>LPCVPFSVAKSVKSLYLGRMFSGTPVIRLRFKRLQPTRLVAEFDFRTFDPEGILLFAGGHQDSTWIVLALRAGRLELQLRYNGVGRVTSSGPVINHGMWQTISVEELARNLVIKVNRDAVMKIAVAGDLFQPERGLYHLNLTVGGIPFHEKDLVQPINPRLDGCMRSWNWLNGEDTTIQETVKVNTRMQCFSVTERGSFYPGSGFAFYSLDYMRTPLDVGTESTWEVEVVAHIRPAADTGVLFALWAPDLRAVPLSVALVDYHSTKKLKKQLVVLAVEHTALALMEIKVCDGQEHVVTVSLRDGEATLEVDGTRGQSEVSAAQLQERLAVLERHLRSPVLTFAGGLPDVPVTSAPVTAFYRGCMTLEVNRRLLDLDEAAYKHSDITAHSCPPVEP[2x];>ESPFVSNPGNITGARGLTGTLRCQLQVQGEPPEVHWLRDGQILELVDSTQTQVPLGEDEQGDWIVASQLRITSLQ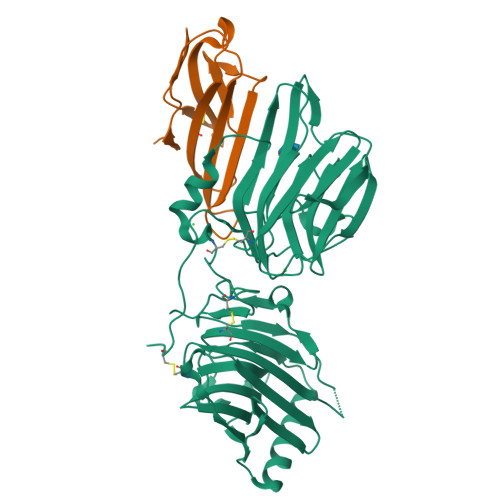LSDTGQYQCLVFLGHQTFVSQPGYVRL[2x]> ANSTAELEELLMQRSLTDPQLQAAAAAAADFRILPDATVIKIGGQSVIDRGRAAVYPLVDEIVAARKNHKLLIGTGAGTRARHLYSIAAGLGLPAGVLAQLGSSVADQNAAMLGQLLAKHGIPVVGGAGLSAVPLSLAEVNAVVFSGMPPYKLWMRPAAEGVIPPYRTDAGCFLLAEQFGCKQMIFVKDEDGLYTANPKTSKDATFIPRISVDEMKAKGLHDSILEFPVLDLLQSAQHVREVQVV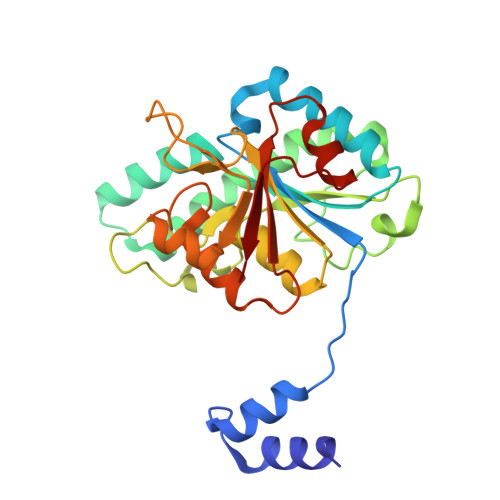NGLVPGNLTRALAGEHVGTIITAS> PLTEIQVESYKKALQADVPPEKRENVGIQAAFKETFPIEEGDKGKGGLVLDFLEYRIGDPPFSQDECREKDLTYQAPLYARLQLIHKDTGLIKEDEVFLGHLPLMTEDGSFIINGADRVIVSQGGRTVGELMADQFRVGLARLARGVRERMVMGSPDTLTPAKLVNSRPLEAALREFFSRSQLS;> EFRPGDKVVLPPYGVGVVAGIAQRSVSGVSRAYYQVDFPGSRSKAYVPVEAPHSVGLRKALAPEEVPVILDLLKNGRMPLPKQWAARHRKTSEILADGNPYRIAQMAGQLRAWEVERGLPD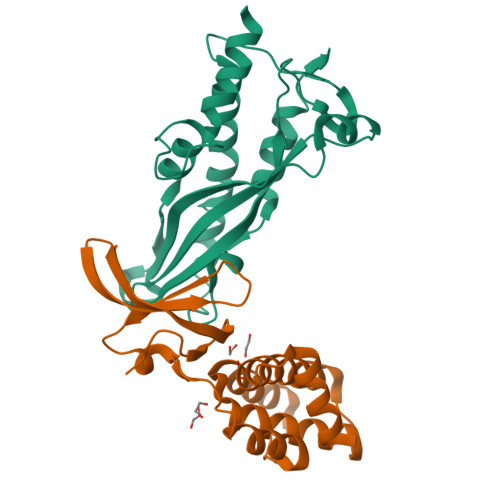LDRQALRRAIHLLAEEVAQSLEITVQEAKRLFEEAWG> NQFYSVEVGDSTFTVLKRYQNLKPIGSGAQGIVCAAYDAVLDRNVAIKKLSRPFQNQTHAKRAYRELVLMKCVNHKNIISLLNVFTPQKTLEEFQDVYLVMELMDANLCQVIQMELDHERMSYLLYQMLCGIKHLHSAGIIHRDLKPSNIVVKSDCTLKILDFGLARTAGTSFMMTPYVVTRYYRAPEVILGMGYKENVDIWSVGCIMGEMVRHKILFPGRDYIDQWNKVIEQLGTPCPEFMKKL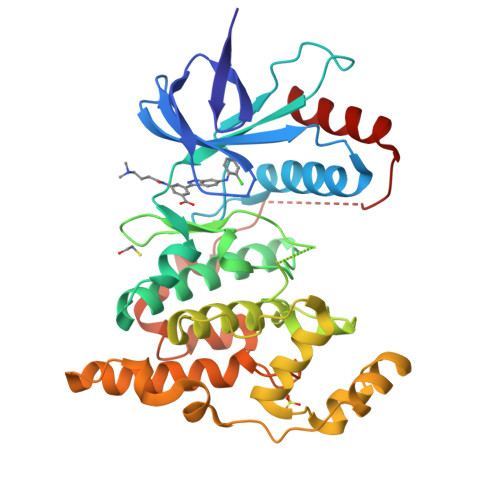QPTVRNYVENRPKYAGLTFPKLFPDSLFPADSEHNKLKASQARDLLSKMLVIDPAKRISVDDALQHPYINVWYDPAEVEAPPPQIYDKQLDEREHTIEEWKELIYKEVMN> MAATAAEAVASGSGEPREEAGALGPAWDESQLRSYSFPTRPIPRLSQSDPRAEELIENEEPVVLTDTNLVYPALKWDLEYLQENIGNGDFSVYSASTHKFLYYDEKKMANFQNFKPRSNREEMKFHEFVEKLQDIQQRGGEERLYLQQTLNDTVGRKIVMDFLGFNWNWINKQQGKRGW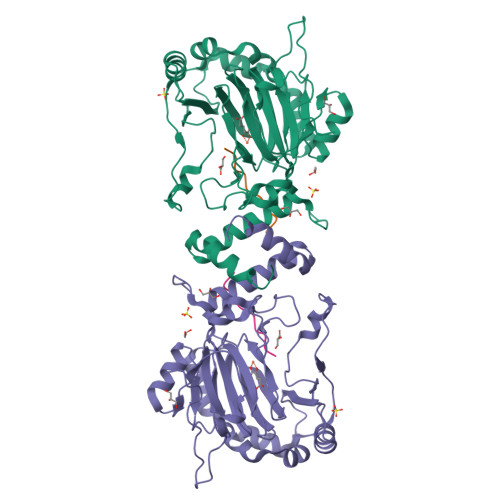GQLTSNLLLIGMEGNVTPAHYDEQQNFFAQIKGYKRCILFPPDQFECLYPYPVHHPCDRQSQVDFDNPDYERFPNFQNVVGYETVVGPGDVLYIPMYWWHHIESLLNGGITITVNFWYKGAPTPKRIEYPLKAHQKVAIMRNIEKMLGEALGNPQEVGPLLNTMIKGRYN;> RSDAAKRLLEASADANIQDN>MIASGGFRKYIAITGRRNVGKSSFMNALIGQEVSIVSNVAGTTTDPVFKSMELSPVGPITLIDTPGLDDVGELGIKRIKKAKKSLYRADCGILIVDDIPGNFEEQIIKLFKELEIPYFIAINKIDTIDHENIEKEYKKYNVPILKVSALKKIGFEKIGKTINSILPKDDEIPYLSDLIDGGDLVILVVPIDLGAPKGRLIMPQVHAIREGLDREALVLVVKERELRYAIENIGIKPRLVVTDSQSVMKVVSDVPEDIDLTTFSILE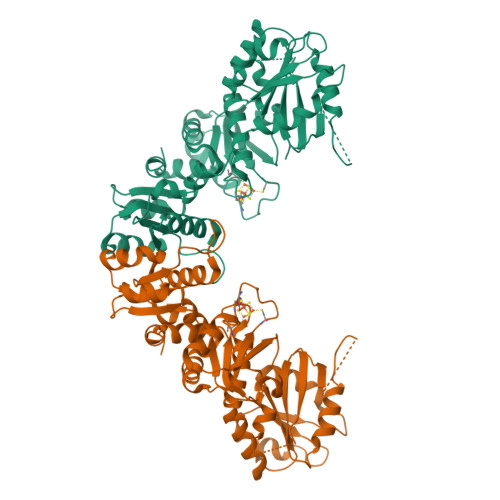SRYRGDLEYFVESVKAVENLKDGDTVIIMEGCTHRPLTEDIGRVKIPRWLTNHTGAALNLKVWAGVDMPELSEIEDAKLIIHCGGCVMNRNNMMRRVRMFKRLNIPMTNYGVVISYLHGVLERAIKPLMR[4x]> MIKNLEIQMLKPENNLEKEAWEINNPAMCSYMLWIATLAYYQKQKEPIHPSRLFCLFPFILYSDTRNVLLSSKGSLKSYLAKFSNSKAISGDIPLSIHFRIDIQKNK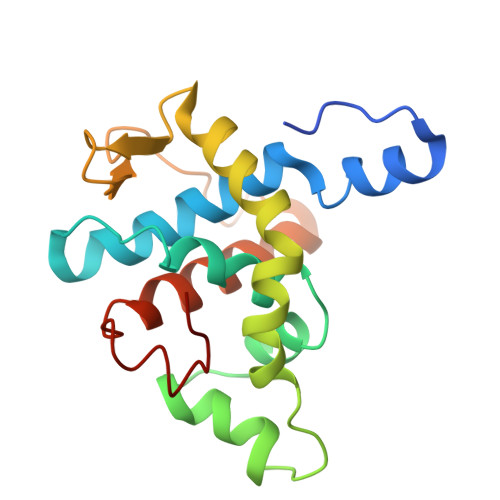TLDALIVAFDSGLLVIDSDSGLIKPNVSIKPLPNSKLTDTIKELVYCSTKIGRWLSEMTNQDLARDLKVIF> GSAKDPMPKSEIRKLLQEIKKQVDNPGNSSTTEIKKMASEA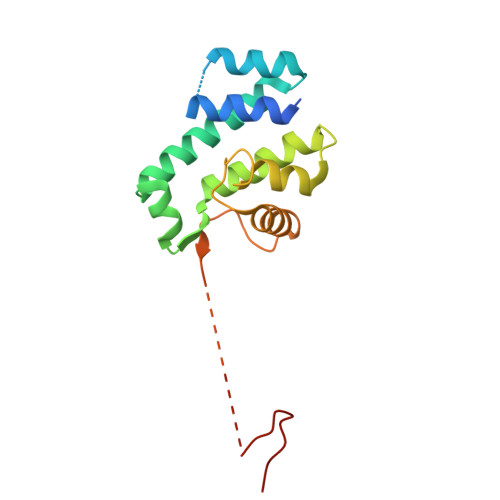GIDEQTAEEIYHLLTEFYQAVEEHGGIEKYMHSNISWLKIELELLSACYQIAILEDMKVLDISEMLSLNDLRIFPKTPSQLQNTYYKLKKELIQVEDIPKNKPGRKRKTQKNTKKEKTNIFGKVVPA> DEEAL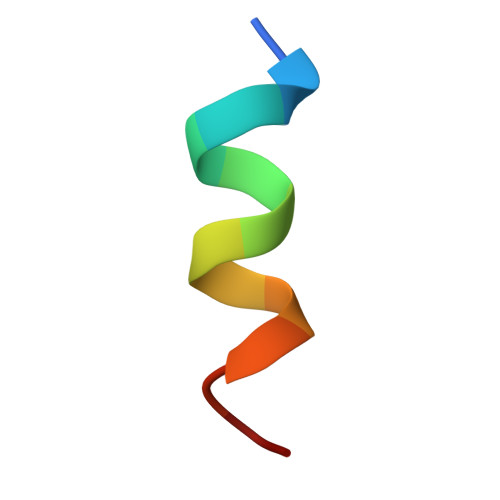KQLAEWVS> GSKVVKFSYMWTINNFSFCREEMGEVIKSSTFSSGANDKLKWCLRVNPKGLDEESKDYLSLYLLLVSCPKSEVRAKFKFSILNAKGEETKAMESQRAYRFVQGKDWGFKKFIRRGFLLDEANGLLPDDKLTLFCEVSVVQDSVNISGQNTMNMVKVPECRLADEL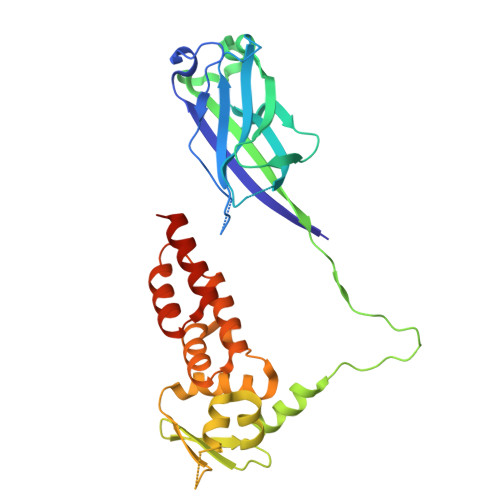GGLWENSRFTDCCLCVAGQEFQAHKAILAARSPVFSAMFEHEMEESKKNRVEINDVEPEVFKEMMCFIYTGKAPNLDKMADDLLAAADKYALERLKVMCEDALCSNLSVENAAEILILADLHSADQLKTQAVDFINYHATDVLETSG> RTTRDDLINGNSASCADVIFIYARGSTETGNLGTLGPSIASNLESAFGKDGVWIQGVGGAYRATLGDNALPRGTSSAAIREMLGLFQQANTKCPDATLIAGGYSLGAALAAASIEDLDSAIRDKIAGTVLFGYTKNLQNRGRIPNY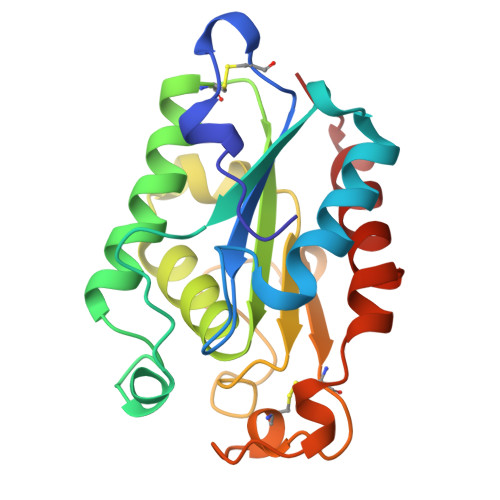PADRTKVFCNTGDLVCTGSLIVAAPHLAYGPDARGPAPEFLIEKVRAVRGS> MEWKDIKGYEGHYQVSNTGEVYSIKSGKTLKHQIPKDGYHRIGLFKGGKGKTFQVHRLVAIHFCEGYEEGLVVDHKDGNKDNNLSTNLRWVTQKINVE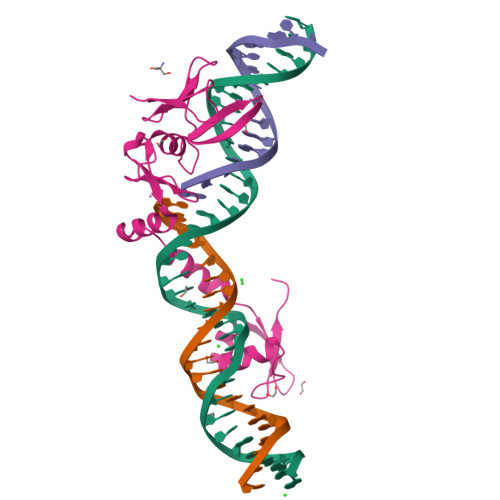NQMSRGTLNVSKAQQIAKIKNQKPIIVISPDGIEKEYPSTKCACEELGLTRGKVTDVLKGHRIHHKGYTFRYKLNG>[6x]SNASISMANPIKTYHLSNLTQTELLSLKSRPRIDFSSVFDIVNPIVDDVHAHGDAAVKQYTSKFDKVDLENIVELVSDLPDPVLDPAIKEAFDVAYSNIYAFHAAQKSPEKSVENMKGVQCKRVARSINSVGLYVPGGTAVLPSTALM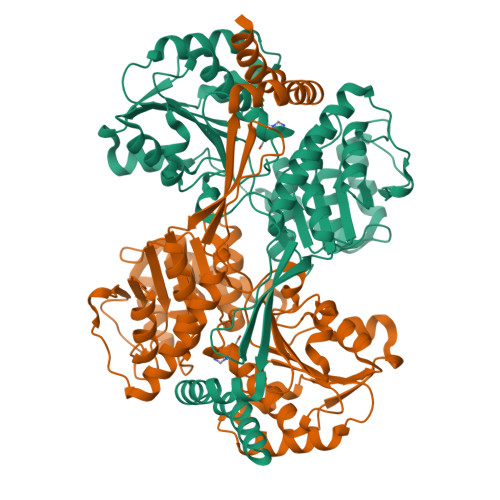LAVPAQIAGCKTIVLANPPTRDGTTCKEVLYCAKKAGVTHLLKAGGAQAISAMAWGTETCPKVEKIFGPGNQYVTAAKMILQNSEAMVSIDMPAGPSEVLVIADKHAIPSHVAADLLSQAEHGPDSQVVLVIAGDGVDQNAIQEEVSKQCQSLPRGEFAAKALSHSFIVHARDMLEAITFSNMYAPEHLIINVKDAEKWESFIENAGSVFLGSWTPESVGDYASGTNHVLPTYGYARMYSGVSLDSFLKYITVQSLTEEGLRKLGPYVETMAEVEGLEAHKRAVTLRLQDIEARQVSR> 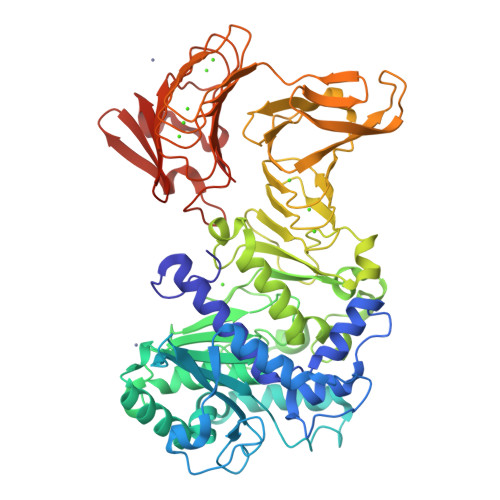MGVYDYKNFGTADSKALFSDAMAITLYSYHNLDNGFAAGYQHNGFGLGLPATLVTALLGGTDSQGVIPGIPWNPDSEKLALDAVKKAGWTPITASQLGYDGKTDARGTFFGEKAGYTTAQVEILGKYDAQGHLTEIGIAFRGTSGPRENLILDSIGAVINDLLAAFGPKDYAKNYVGEAFGNLLNDVVAFAKANGLSGKDVLVSGHSLGGLAVNSMADLSGGKWGGFFADSNYIAYASPTQSSTDKVLNVGYENDPVFRALDGSTFTGASVGVHDAPKESATDNIVSFNDHYASTAWNLLPFSILNIPTWISHLPTAYGDGMNRIIESKFYDLTSKDSTIIVANLSDPARANTWVQDLNRNAETHKGSTFIIGSDSNDLIQGGSGNDYLEGRAGNDTFRDGGGYNVILGGAGNNTLDLQKSVNTFDFANDGAGNLYVRDANGGISITRDIGSIVTKEPGFLWGLFKDDVTHSVTASGLKVGSNVTQYDASVKGTNGADTLKAHAGGDWLFGLDGNDHLIGGVGNDVFVGGAGNDLMESGGGADTFLFNGAFGQDRVVGFTSNDKLVFLGVQGVLPNDDFRAHASMVGQDTVLKFGGDSVTLVGVALNSLSADGIVIA>[2x]MNHLGKTEVFLNRFALRPLNPEELRPWRLEVVLDPPPGREEVYPLLAQVARRAGGVTVRMGDGLASWSPPEVLVLEGTLARMGQTYAYRLYPKGRRPLDPKDPGERSVLSAL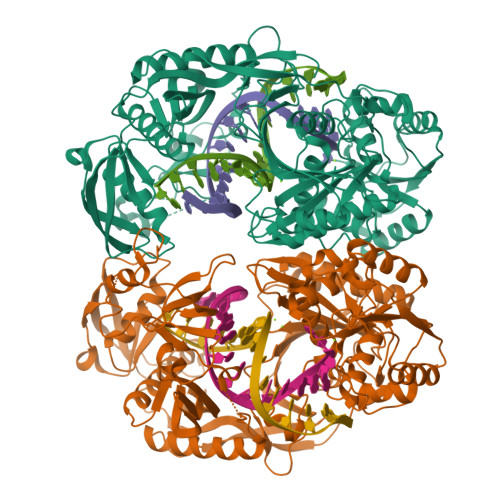ARRLLQERLRRLEGVWVEGLAVYRREHARGPGWRVLGGAVLDLWVSDSGAFLLEVDPAYRILCEMSLEAWLAQGHPLPKRVRNAYDRRTWELLRLGEEDPKELPLPGGLSLLDYHASKGRLQGREGGRVAWVADPKDPRKPIPHLTGLLVPVLTLEDLHEEEGSLALSLPWEERRRRTREIASWIGRRLGLGTPEAVRAQAYRLSIPKLMGRRAVSKPADALRVGFYRAQETALALLRLDGAQGWPEFLRRALLRAFGASGASLRLHTLHAHPSQGLAFREALRKAKEEGVQAVLVLTPPMAWEDRNRLKALLLREGLPSQILNVPLREEERHRWENALLGLLAKAGLQVVALSGAYPAELAVGFDAGGRESFRFGGAACAVGGDGGHLLWTLPEAQAGERIPQEVVWDLLEETLWAFRRKAGRLPSRVLLLRDGRVPQDEFALALEALAREGIAYDLVSVRKSGGGRVYPVQGRLADGLYVPLEDKTFLLLTVHRDFRGTPRPLKLVHEAGDTPLEALAHQIFHLTRLYPASGFAFPRLPAPLHLADRLVKEVGRLGIRHLKEVDREKLFFV> MSSSSYRDSYFQYRHLPAPHHILYAEWNQDILALPDEVANITMAMKDNTRTDAEEGRAPQDGERNSNVRESAQGKALMTSEQNSNRYWNSFHDEDDWNLFNGMELESNGVVTFAGQAFDHSLNGGTNSRNDGANEPRKETITGSIFDRRITQL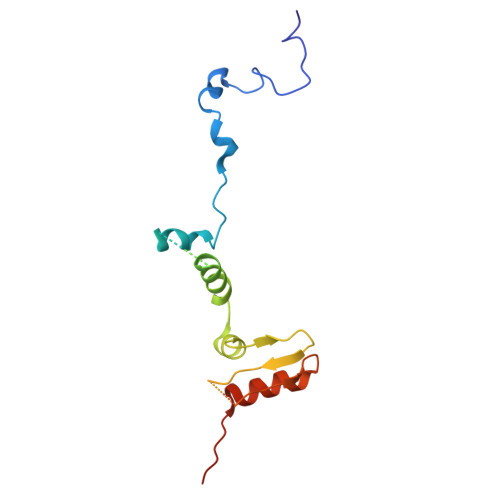AYARNNGWHELALPQSR> PQLEDFPALIKQASL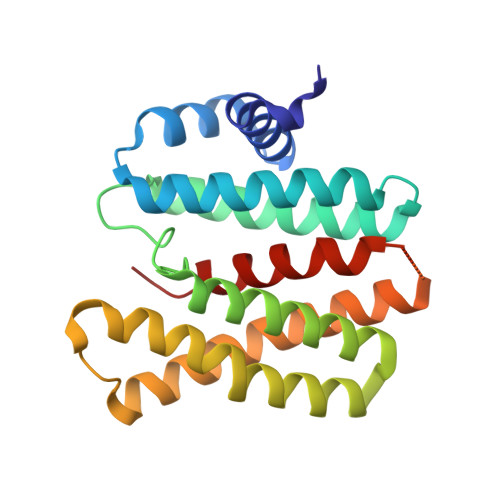DALFKCGKDAEALKEVFTNSNNVAGKKAIMEFAGLFRSALNATSDSPEAKTLLMKVGAEYTAQIIKDGLKEKSAFGPWLPETKKAEAKLENLEKQLLDIIKNNTGGELSKLSTNLVMQEVMPYIASCIEHNFGCTLDPLTRSNLTHLVDKAAAKAVEALDMCHQKLTQEQGTSVGREARHLEMQTLIPLLLRNVFAQIPA>TDKERFIASLMARMSNAEKIGQLRLVSVGADHPKEALMADIRAGKVGAIFNTVTRPDIRAMQDQVRHSRLKIPLFHAYDVAHGHRTIFPISLGLAASWDPEVVARSARISALEASADGLDMSFSPMVDITRDARWGRVSEGFGEDTYLTSLLSGVMVRAYQGSNLAAPDSIMAAVKHFALYGAAEGGRDYNTVDMSLPRMFQDYLPPYKAAVDAGAGAVMVSLNTINGVPATANRWLLTDLLRQQWGFKGLTISNHGAVKELIKHGLAGNERDATRLAIQAGVDMNMNDDLYSTWLPKLLAAGEIDQADIDRACRDVLAAKYDLGLFADPYRRLGKPDDPPFDTNAESRLHRQAAREVAREGLVLLKNRDGLLPLKKQGRIAVIGPLAKSQRDVIGSWSAAGVPRQAVTVYQGLANAVGERATLLYAKGANVSGDQAILDYLNSYNPEVEVDPRSAEAMLEEALRTARDADLVVAVVGESQGMAHEASSRTDLRIPASQRRLLKALKATGKPLVLVLMNGRPLSLGWEQ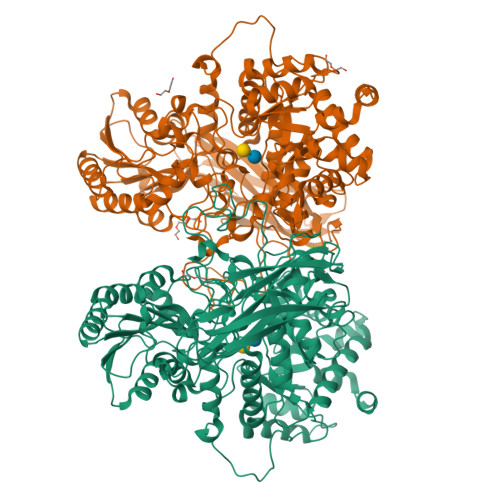ENADAILETWFSGTEGGNAIADVLFGEHNPSGKLTMSFPRSVGQVPVYYNHLNTGRPMDHDNPGKYTSRYFDEANGPLYPFGYGLSYTEFSLSPLRLSSERLARGATLEARVTLSNSGKRAGATVVQLYLQDPVASLSRPVKELRGFRKVMLEPGESREIVFRLGEADLKFYDSQLRHTAEPGEFKVFVGLDSAQTESRSFTLL[2x]>[2x]MEWSQIFHDITTKHDFKAMHDFLEKEYSTAIVYPDRENIYQAFDLTPFENIKVVILGQDPYHGPNQAHGLAFSVQPNAKFPPSLRNMYKELADDIGCVRQTPHLQDWAREGVLLLNTVLTVRQGEANSHRDIGWETFTDEIIKAVSDYKEHVVFILWGKPAQQKIKLIDTSKHCIIKSVHPSPLSAYRGFFGSKPYSKANTYLESVGKSPINWCESEALEHHHHHH;>[2x]MYKNIEDLNKFASKILETEISFEESITFTPDEVEENIGEKPNRDKICHSTSLEDGRVIMLLTELEPNYTPWKLLELEEDGFKELYSKSI

Ung (family 1 of the UDG superfamily) is the most prevalent form of UDG and removes uracil bases, regardless of their state of base pairing or sequence context, via the cleavage of the glycosyl bond attaching them to the deoxyribose. Ung inhibitors (which are interchangeably referred to herein as UngIns) are DNA mimetic proteins utilising charge-based alignment with the Ung DNA binding cleft to dock Ung. Docking promotes the hydrophobic sequestration of the sidechain of the apical residue in the Ung DNA minor groove binding loop, which is essentially irreversible under biological conditions, to inhibit Ung. UngIn protein structures described to date fall into one of three observed folds: Ugi/SAUGI (note that Ugi and SAUGI share the same protein fold at ~12% sequence residue identity), p56, and Vpr; yet, within each fold, type there is pronounced sequence plasticity, to the extent that the unambiguous identification of an Ung inhibitor in any genome is rarely straightforward.

The weakest homolog is encoded by Bacillus phage vB_BpuM-BpSp (locus_tag = “Bp8pS_259”; accession number ALN97938) and 32% of its identity is composed of Ugi (as encoded by Bacillus phages AR9, PBS1 and PBS2). This sequence (referred to henceforth as Ugi-2) was biochemically and biochemically/structurally validated to act as an UngIn. Ugi and Ugi-2 variants show structural conservation (RMSD = 1.343 Å) despite low sequence identity (32%). Although not identical, the negative charge distribution on the surface of each Ugi variant effectively mimics the negative charge distribution of phosphate groups on Ung-bound DNA; in addition, the grooves of DNA are mimicked by depressions on the surface of each Ugi variant. Ugi-2 has 21 acidic residues in its primary sequence, while PBS1 Ugi has 18 acidic residues. There are only eight positions of conserved negatively charged residues between the two Ugi sequence variants, of which, five are within the Ung-binding β-strand 1 and α-helix 2 in a 12aa span. A PROSITE pattern of E-X(6)-[ED]-[ED]-X-[ED]-[ED] may thus be defined for these Ugi variants. The Ung-sequestering hydrophobic pocket of PBS1 Ugi is formed by eight residues, of which, only four are identical in Ugi-2. This provides important data on tolerated variations, including the essential residues that perform Ung inhibition. Sequence diversity is not limited to the loops and other flexible secondary structures.>ALYEDPPDQKTSPSGKPATLKICSWNVDGLRAWIKKKGLDWVKEEAPDILCLQETKCSENKLPAELQELPGLSHQYWSAPSDKEGYSGVGLLSRQAPLKVSYGIGDEEHDQEGRVIVAEFDSFVLVTAYVPQAGRGLVRLEYRQRWDEAFRKFLKGLASRKPLVLCGDLNVAHEEIDLRNPKGNKKNAGFTPQERQGFGELLQAVPLADSFRHLYPNTPYAYTFWTYMMNARSKNVGWRLDYFLLSHSLLPALCDSKIRSKALGSDHCPITLYLAL[2x]

AP sites are then processed by apurinic/apyrimidinic endonuclease 1 (APE1), which cleaves the phosphodiester DNA backbone at the 5′ end of the AP site using its endonuclease activity. Upon binding an AP site, APE1 flips the AP site out of the DNA double helix and into an extrahelical position within the compact APE1 active site. In the human APE1 substrate complex, N174 is within hydrogen bonding distance of N212 and the AP site bridging oxygen (O5) and deoxyribose sugar oxygen (O4). To assess the role of N174 during APE1 catalysis, we rationally designed four mutations of N174: N174A, N174D, N174Q, and N174K.

The APE1N174Q mutant had a kobs of 2.9 ± 0.3 s−1, corresponding to a 290-fold reduction in kobs compared to APE1WT. We crystallized the APE1N174Q mutant bound to a 21-mer dsDNA oligo containing a centrally located AP site analog, THF. In these crystals, the backbone has been cleaved by APE1 resulting in a product complex that diffracted to 2.25 Å resolution in the P43 space group. The crystal form of the APE1N174Q mutant product complex contains two nearly identical APE1N174Q:DNA complexes (RMSD = 0.452 of 2329 atoms). The AP site is positioned in the APE1N174Q mutant active site with clear density for the cleaved DNA backbone and a bound Mg2+ ion. As in both the APE1N174A and APE1N174D mutant product complexes, residue N212 failed to undergo the rotameric shift observed in the APE1WT product complex structure and remains in the substrate conformation. We did observe one additional change not present in either the APE1N174A or APE1N174D mutant product complexes at residue D308, which adopts a different rotameric confirmation than in APE1WT. In the APE1N174Q mutant, the 3′ hydroxyl terminus shifts 2.6 Å away from the mutant active site. Comparing APE1WT to the APE1N174Q mutant indicates that this shift in the 3′ hydroxyl terminus arises to allow the mutant active site to accommodate the extra side chain length of N174Q and prevent a clash between N174Q and the sugar moiety of the 3′ terminus. We suggest that this difference likely results from a subtle displacement of the DNA within the APE1N174Q mutant active site to accommodate the added side chain length of N174Q as observed in our product complex.>[3x]MRRAVIIPARLGSTRLKEKPLKNLLGKPLIRWVVEGLVKTGERVILATDSER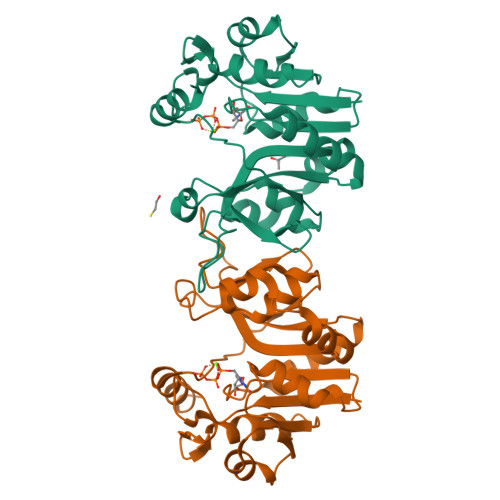VKEVVEDLCEVFLTPSDLPSGSDRVLYVVRDLDVDLIINYQGDEPFVYEEDIKLIFRELEKGERVVTLARKDKEAYERPEDVKVVLDREGYALYFSRSPIPYFRKNDTFYPLKHVGIYGFRKETLMEFGAMPPSKLEQIEGLEQLRLLENGIKIKVLITENYYHGVDTEEDLKIVEEKLKNL> GPHMPDPAAHLPFFY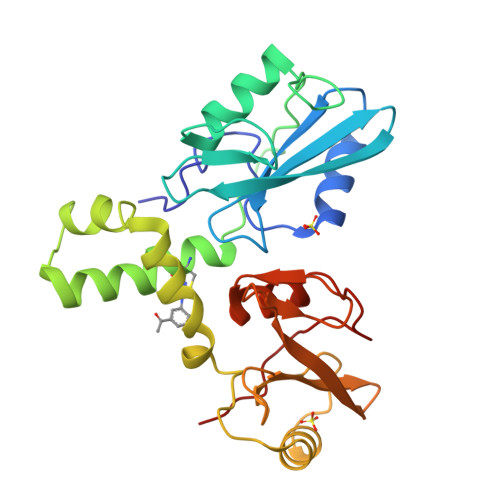GSISRAEAEEHLKLAGMADGLFLLRQCLRSLGGYVLSLVHDVRFHHFPIERQLNGTYAIAGGKAHCGPAELCEFYSRDPDGLPCNLRKPCNRPSGLEPQPGVFDCLRDAMVRDYVRQTWKLEGEALEQAIISQAPQVEKLIATTAHERMPWYHSSLTREEAERKLYSGAQTDGKFLLRPRKEQGTYALSLIYGKTVYHYLISQDKAGKYCIPEGTKFDTLWQLVEYLKLKADGLIYCLKEACPNSSA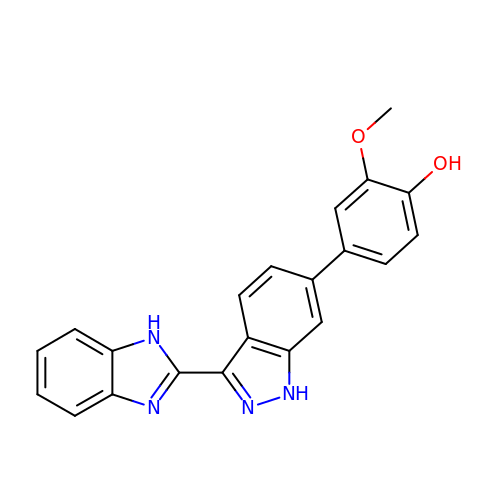4-[3-(1H-BENZIMIDAZOL-2-YL)-1H-INDAZOL-6-YL]-2-METHOXYPHENOL | C21 H16 N4 O2 | GYPHGCGOSZJXOT-UHFFFAOYSA-N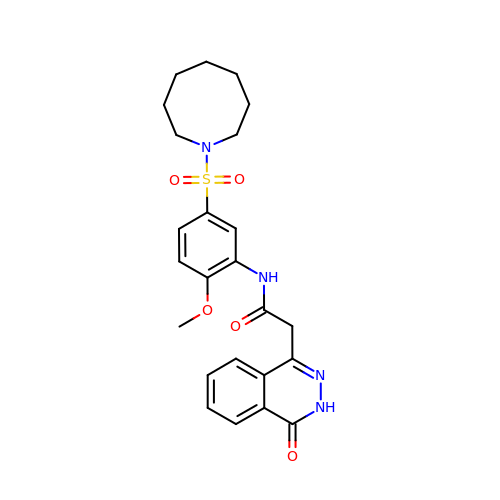~{N}-[5-(azocan-1-ylsulfonyl)-2-methoxy-phenyl]-2-(4-oxidanylidene-3~{H}-phthalazin-1-yl)ethanamide | C24 H28 N4 O5 S | ZQSQGRGBMUBDMZ-UHFFFAOYSA-N>[6x]MKTNYEIRYAAHPEDAKSYDTTRIRRDFLIEKIFVPNEVNMVYSMYDRMVVGGALPVGEVLTLEAIDPLKAPFFLTRREMGIYNVGGPGIVKAGDAEFELDYKEALYLGSGDRVVTFESKDAAHPAKFYFNSLTAHRNYPDRKVTKADAVVAEMGSLEGSNHRNINKMLVNQVLPTCQLQMGMTELAPGSVWNTMPAHVHSRRMEAYFYFEIPEDHAICHFMGEVGE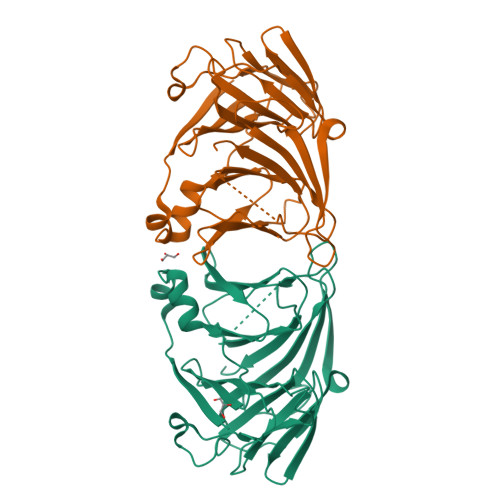TRHVWMKGDQAVLSPEWSIHSAAATHNYTFIWGMGGENLDYGDQDFSLITDLKLEHHHHHH>GSCQVIGMYDYTAQNDDELAFSKGQIINVLNKEDPDWWKGEVSGQVGLFPSNYVKLTTDMDPSQQWCSDLHLLDMLTPTERKRQGYIHELIVTEENYVNDLQLVTEIFQKPLTESELLTEKEVAMIFVNWKELIMCNIKLLKALRVRKKMSGEKMPVKMIGD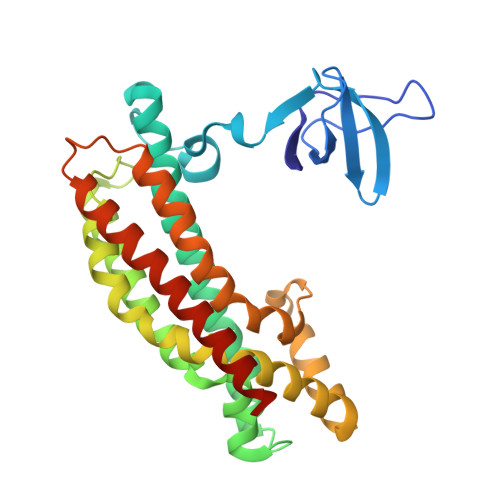ILSAQLPHMQPYIRFCSCQLNGAALIQQKTDEAPDFKEFVKRLAMDPRCKGMPLSSFILKPMQRVTRYPLIIKNILENTPENHPDHSHLKHALEKAEELCSQVNEGVREKENSDRLEWIQA[2x]N-hydroxy-2-{4-[3-(4-{[(2S)-2-hydroxy-3,3-dimethylbutyl]oxy}-3-methylphenyl)pentan-3-yl]-2-methylphenoxy}acetamide 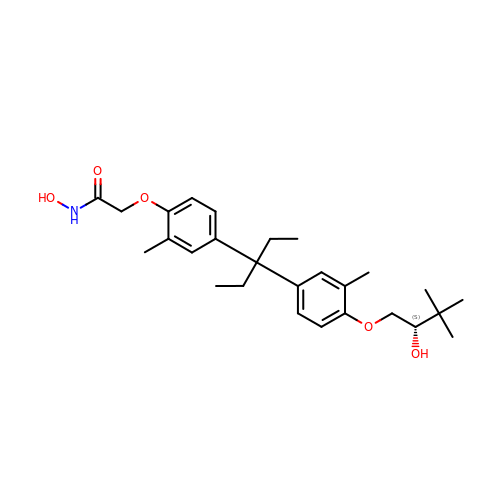| C27 H39 N O5 | HLEDBIQBAUIWNJ-XMMPIXPASA-N>[2x]MKHHHHHHPMTTKQWGITPPISTAPATEQENALNTALINELKNQNLFESPAESEKRVKVLDELQQITTEFVKKVSLAKHMNEKMANEAGGKIFTYGSYRLGVYGPGSDIDTLVVVPKHVSRDNFFQDLEPMLREREEVTDLAAVPDAYVPIIKFKFLGISIDLIFARLSVPRVPRDLELSDNNLLKGVEERCVLSLNGTRVTDQILQLVPNRAVFKHALRAIKFWAQRRAIYANVVGFPGGVAWAMMVARICQLYPNAVSSVIVAKFFRILHQWNWPQPILLKPIEDGPLQVRIWNPKLYPSDKAHRMPIITPAYPSMCATHNITLSTQTIILREMVRAGEIADQIMVKALPWSALFQKHDFFHRYKHYLTITAAAKTAEAQLKWAGLVESKLRHLVTRLELVDAIALAHPFNKGFDKVYNCSSEEEAQQVASGVTLEVAYESTDHEKLANDTVNEEKADNTESKADGSENGEKQIFPVYTTTCYIGLELEKKKGHPIKRLDISWPTQEFYELCKKWDKYDDTLMNVFIKNTKNTALPDEVFEPGEERPKA

The S. pombe orthologue of the human PAXT connection, Mtl1-Red1 Core (MTREC), is an eleven-subunit complex that targets cryptic unstable transcripts (CUTs) to the nuclear RNA exosome for degradation. It encompasses the canonical poly(A) polymerase Pla1, responsible for polyadenylation of nascent RNA transcripts as part of the cleavage and polyadenylation factor (CPF/CPSF). We report crystal structures of Pla1 in its apo form and in complex with Red1. Taken together, our data reveal the molecular details of recruitment of Pla1 by Red1 which leads to hyperadenylation of CUTs, serving as a signal for exosome-mediated target degradation.

We expressed, purified and performed crystallisation trials with the full-length (Pla1FL) and a C-terminal truncation (Pla1Δ14) of Pla1. Both constructs readily crystallised under a variety of conditions within 2–4 days. A comparison of our crystal structures of Pla1FL and Pla1Δ14 shows that the individual domains have undergone significant movements. An alignment based on the middle domains illustrates that the N-terminal has a modest rotation of 2.95° with a 1.13 Å displacement, while the C-terminal RRM domain has a more pronounced rotation of 9.8° and 2.26 Å displacement.(4-methylphenyl) 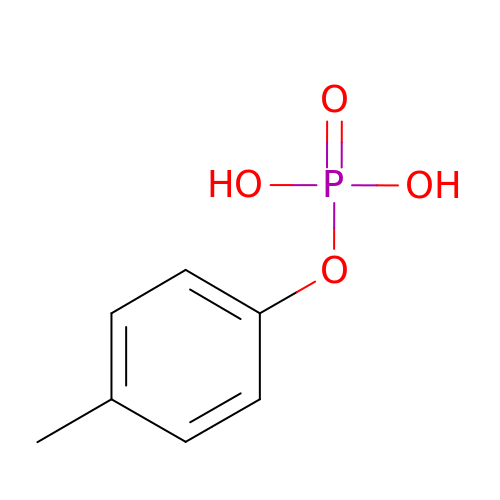dihydrogen phosphate | C7 H9 O4 P | JNUCNIFVQZYOCP-UHFFFAOYSA-N> MSDNRRRRREEDDSDSENELPPSSPQQHFRGGMNPVSSPIGSPDMINPEGDDNEVDDVPDIDEVEEQMNEVDLMDDNMYEDYAADHNRDRYDPDQVDDREQQELSLSERRRIDAQLNERDRLLRNVAYIDDEDEEQEGAAQLDEMGLPVQRRRRRRQYEDLENSDDDLLSDMDIDPLREELTLESLSNVKANSYSEWITQPNVSRTIARELKSFLLEYTDETGRSVYGARIRTLGEMNSESLEVNYRHLAESKAILALFLAKCPEEMLKIFDLVAMEATELHYPDYARIHSEIHVRISDFPTIYSLRELRESNLSSLVRVTGVVTRRTGVFPQLKYVKFNCLKCGSILGPFFQDSNEEIRISFCTNCKSKGPFRVNGEKTVYRNYQRVTLQEAPGTVPPGRLPRHREVILLADLVDVSKPGEEVEVTGIYKNNYDGNLNAKNGFPVFATIIEANSIKRREGNTANEGEEGLDVFSWTEEEEREFRKISRDRGIIDKIISSMAPSIYGHRDIKTAVACSLFGGVPKNVNGKHSIRGDINVLLLGDPGTAKSQILKYVEKTAHRAVFATGQGASAVGLTASVRKDPITKEWTLEGGALVLADKGVCLIDEFDKMNDQDRTSIHEAMEQQSISISKAGIVTTLQARCSIIAAANPNGGRYNSTLPLAQNVSLTEPILSRFDILCVVRDLVDEEADERLATFVVDSHVRSHPENDEDREGEELKNNGESAIEQGEDEINEQLNARQRRLQRQRKKEEEISPIPQELLMKYIHYARTKIYPKLHQMDMDKVSRVYADLRRESISTGSFPITVRHLESILRIAESFAKMRLSEFVSSYDLDRAIKVVVDSFVDAQKVSVRRQLRRSFAIYTLGH;> MKRRWKKNFIAVSAANRFKKISSSGALENLYFQGEA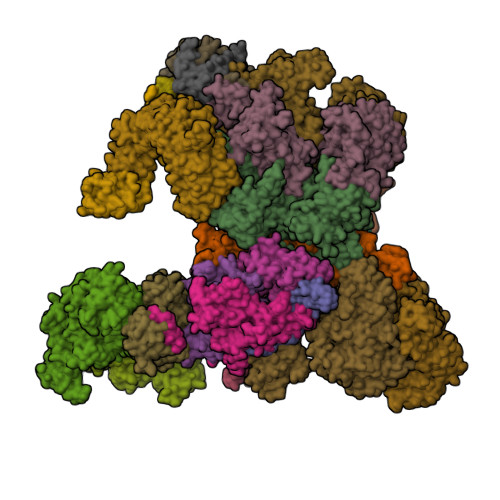PVMEGSTGFDGDATTFFAPDAVFGDRVRRFQEFLDTFTSYRDSVRSIQVYNSNNAANYNDDQDDADERDLLGDDDGDDLEKEKKAASSTSLNILPHRIIISLDDLREFDRSFWSGILVEPAYFIPPAEKALTDLADSMDDVPHPNASAVSSRHPWKLSFKGSFGAHALSPRTLTAQHLNKLVSVEGIVTKTSLVRPKLIRSVHYAAKTGRFHYRDYTDATTTLTTRIPTPAIYPTEDTEGNKLTTEYGYSTFIDHQRITVQEMPEMAPAGQLPRSIDVILDDDLVDKTKPGDRVNVVGVFKSLGAGGMNQSNSNTLIGFKTLILGNTVYPLHARSTGVAARQMLTDFDIRNINKLSKKKDIFDILSQSLAPSIYGHDHIKKAILLMLMGGVEKNLENGSHLRGDINILMVGDPSTAKSQLLRFVLNTASLAIATTGRGSSGVGLTAAVTTDRETGERRLEAGAMVLADRGVVCIDEFDKMTDVDRVAIHEVMEQQTVTIAKAGIHTTLNARCSVIAAANPVFGQYDVNRDPHQNIALPDSLLSRFDLLFVVTDDINEIRDRSISEHVLRTHRYLPPGYLEGEPVRERLNLSLAVGEDADINPEEHSNSGAGVENEGEDDEDHVFEKFNPLLQAGAKLAKNKGNYNGTEIPKLVTIPFLRKYVQYAKERVIPQLTQEAINVIVKNYTDLRNDDNTKKSPITARTLETLIRLATAHAKVRLSKTVNKVDAKVAANLLRFALLGEDIGNDIDEEESEYEEALSKRSPQKSPKKRQRVRQPASNSGSPIKSTPRRSTASSVNATPSSARRILRFQDDEQNAGEDDNDIMSPLPADEEAELQRRLQLGLRVSPRRREHLHAPEEGSSGPLTEVGTPRLPNVSSAGQDDEQQQSVISFDNVEPGTISTGRLSLISGIIARLMQTEIFEEESYPVASLFERINEELPEEEKFSAQEYLAGLKIMSDRNNLMVADDKVWRV;> MSQQSSSPTKEDNNSSSPVVPNPDSVPPQLSSPALFYSSSSSQGDIYGRNNSQNLSQGEGNIRAAIGSSPLNFPSSSQRQNSDVFQSQGRQGRIRSSASASGRSRYHSDLRSDRALPTSSSSLGRNGQNRVHMRRNDIHTSDLSSPRRIVDFDTRSGVNTLDTSSSSAPPSEASEPLRIIWGTNVSIQECTTNFRNFLMSFKYKFRKILDEREEFINNTTDEELYYIKQLNEMRELGTSNLNLDARNLLAYKQTEDLYHQLLNYPQEVISIMDQTIKDCMVSLIVDNNLDYDLDEIETKFYKVRPYNVGSCKGMRELNPNDIDKLINLKGLVLRSTPVIPDMKVAFFKCNVCDHTMAVEIDRGVIQEPARCERIDCNEPNSMSLIHNRCSFADKQVIKLQETPDFVPDGQTPHSISLCVYDELVDSCRAGDRIEVTGTFRSIPIRANSRQRVLKSLYKTYVDVVHVKKVSDKRLDVDTSTIEQELMQNKVDHNEVEEVRQITDQDLAKIREVAAREDLYSLLARSIAPSIYELEDVKKGILLQLFGGTNKTFTKGGRYRGDINILLCGDPSTSKSQILQYVHKITPRGVYTSGKGSSAVGLTAYITRDVDTKQLVLESGALVLSDGGVCCIDEFDKMSDSTRSVLHEVMEQQTISIAKAGIITTLNARSSILASANPIGSRYNPNLPVTENIDLPPPLLSRFDLVYLVLDKVDEKNDRELAKHLTNLYLEDKPEHISQDDVLPVEFLTMYISYAKEHIHPIITEAAKTELVRAYVGMRKMGDDSRSDEKRITATTRQLESMIRLAEAHAKMKLKNVVELEDVQEAVRLIRSAIKDYATDPKTGKIDMNLVQTGKSVIQRKLQEDLSREIMNVLKDQASDSMSFNELIKQINEHSQDRVESSDIQEALSRLQQEDKVIVLGEGVRRSVRLNNRV;> MSFDRPEIYSAPVLQGESPNDDDNTEIIKSFKNFILEFRLDSQFIYRDQLRNNILVKNYSLTVNMEHLIGYNEDIYKKLSDEPSDIIPLFETAITQVAKRISILSRAQSANNNDKDPENTSMDTDSLLLNSLPTFQLILNSNANQIPLRDLDSEHVSKIVRLSGIIISTSVLSSRATYLSIMCRNCRHTTSITINNFNSITGNTVSLPRSCLSTIESESSMANESNIGDESTKKNCGPDPYIIIHESSKFIDQQFLKLQEIPELVPVGEMPRNLTMTCDRYLTNKVIPGTRVTIVGIYSIYNSKNGAGSGRSGGGNGGSGVAIRTPYIKILGIQSDVETSSIWNSVTMFTEEEEEEFLQLSRNPKLYEILTNSIAPSIFGNEDIKKAIVCLLMGGSKKILPDGMRLRGDINVLLLGDPGTAKSQLLKFVEKVSPIAVYTSGKGSSAAGLTASVQRDPMTREFYLEGGAMVLADGGVVCIDEFDKMRDEDRVAIHEAMEQQTISIAKAGITTVLNSRTSVLAAANPIYGRYDDLKSPGDNIDFQTTILSRFDMIFIVKDDHNEERDISIANHVINIHTGNANAMQNQQEENGSEISIEKMKRYITYCRLKCAPRLSPQAAEKLSSNFVTIRKQLLINELESTERSSIPITIRQLEAIIRITESLAKLELSPIAQERHVDEAIRLFQASTMDAASQDPIGGLNQASGTSLSEIRRFEQELKRRLPIGWSTSYQTLRREFVDTHRFSQLALDKALYALEKHETIQLRHQGQNIYRSGV;> MSSPFPADTPSSNRPSNSSPPPSSIGAGFGSSSGLDSQIGSRLHFPSSSQPHVSNSQTGPFVNDSTQFSSQRLQTDGSATNDMEGNEPARSFKSRALNHVKKVDDVTGEKVREAFEQFLEDFSVQSTDTGEVEKVYRAQIEFMKIYDLNTIYIDYQHLSMRENGALAMAISEQYYRFLPFLQKGLRRVVRKYAPELLNTSDSLKRSEGDEGQADEDEQQDDDMNGSSLPRDSGSSAAPGNGTSAMATRSITTSTSPEQTERVFQISFFNLPTVHRIRDIRSEKIGSLLSISGTVTRTSEVRPELYKASFTCDMCRAIVDNVEQSFKYTEPTFCPNPSCENRAFWTLNVTRSRFLDWQKVRIQENANEIPTGSMPRTLDVILRGDSVERAKPGDRCKFTGVEIVVPDVTQLGLPGVKPSSTLDTRGISKTTEGLNSGVTGLRSLGVRDLTYKISFLACHVISIGSNIGASSPDANSNNRETELQMAANLQANNVYQDNERDQEVFLNSLSSDEINELKEMVKDEHIYDKLVRSIAPAVFGHEAVKKGILLQMLGGVHKSTVEGIKLRGDINICVVGDPSTSKSQFLKYVVGFAPRSVYTSGKASSAAGLTAAVVRDEEGGDYTIEAGALMLADNGICCIDEFDKMDISDQVAIHEAMEQQTISIAKAGIHATLNARTSILAAANPVGGRYNRKLSLRGNLNMTAPIMSRFDLFFVILDDCNEKIDTELASHIVDLHMKRDEAIEPPFSAEQLRRYIKYARTFKPILTKEARSYLVEKYKELRKDDAQGFSRSSYRITVRQLESMIRLSEAIARANCVDEITPSFIAEAYDLLRQSIIRVDVDDVEMDEEFDNIESQSHAASGNNDDNDDGTGSGVITSEPPADIEEGQSEATARPGTSEKKKTTVTYDKYVSMMNMIVRKIAEVDREGAEELTAVDIVDWYLLQKENDLGSLAEYWEERRLAFKVIKRLVKDRILMEIHGTRHNLRDLENEENENNKTVYVIHPNCEVLDQLEPQDSS;> MSAALPSIQLPVDYNNLFNEITDFLVTFKQDTLSSDATRNENEDENLDAENIEQHLLEKGPKYMAMLQKVANRELNSVIIDLDDILQYQNEKFLQGTQADDLVSAIQQNANHFTELFCRAIDNNMPLPTKEIDYKDDVLDVILNQRRLRNERMLSDRTNEIRSENLMDTTMDPPSSMNDALREVVEDETELFPPNLTRRYFLYFKPLSQNCARRYRKKAISSKPLSVRQIKGDFLGQLITVRGIITRVSDVKPAVEVIAYTCDQCGYEVFQEVNSRTFTPLSECTSEECSQNQTKGQLFMSTRASKFSAFQECKIQELSQQVPVGHIPRSLNIHVNGTLVRSLSPGDIVDVTGIFLPAPYTGFKALKAGLLTETYLEAQFVRQHKKKFASFSLTSDVEERVMELITSGDVYNRLAKSIAPEIYGNLDVKKALLLLLVGGVDKRVGDGMKIRGDINVCLMGDPGVAKSQLLKAICKISPRGVYTTGKGSSGVGLTAAVMKDPVTDEMILEGGALVLADNGICCIDEFDKMDESDRTAIHEVMEQQTISISKAGINTTLNARTSILAAANPLYGRYNPRLSPLDNINLPAALLSRFDILFLMLDIPSRDDDEKLAEHVTYVHMHNKQPDLDFTPVEPSKMREYIAYAKTKRPVMSEAVNDYVVQAYIRLRQDSKREMDSKFSFGQATPRTLLGIIRLSQALAKLRLADMVDIDDVEEALRLVRVSKESLYQETNKSKEDESPTTKIFTIIKKMLQETGKNTLSYENIVKTVRLRGFTMLQLSNCIQEYSYLNVWHLINEGNTLKFVDDGTMDTDQEDSLVSTPKLAPQTTASANVSAQDSDIDLQDA;> MYGDLGNKLVLEAKRTKQLYARSNQDVNLPMYHEDIIRNILKEVSNLRKNTEYLKEQQQLGMLDDKVAKCQYFVTLLCMERNKRCLLAYQRLRTDILDSMAWNNNGLDLMSSITFSQQDTNNLSHQEQEYLKEYCDLITDLKSGDLVDIDLSGSLVPPSDVFIDVRVLKDAGEIQTEYGVFNLIKDSQFFVRQSDVERLIQQGYLQKI;> MSLPAHLQQTFSPEEIQFIVENEPIKIFPRITTRQKIRGDDRGTGNHTRWQLITTDDKALNNMVAMRSTEVVLWIALLLKQQSKCSIVAPQWLTTKELDRKIQYEKTHPDRFSELPWNWLVLARILFNKAKDDFHDPIHELRGKIQDLREIRQIKVLKGLKYLNESHLQLDNLSLLEINELRPFITEIMDKLREIHTASLTAGTENDEEEFNI;> MGYYDIDDVLADGTEFPCKFQYDIPGLGYLENNPGRPITKNTKLNLPLWLARILAIVGGDEALVDEEPVPFVELLPPDMFSTKVMNAIKTDPVALDLHSINSHFFSLAIKWIMLFSEKELANVVSELLLQRAQELNHHASSLSIDLNADSTGKNSANTNIATSTFLLKLEEMEKEIYKKSHESYKDTKRWMFKK;> MDINIDDILAELDKETTAVDSTKITQGSSSTTHRDANTIVGSSLDLNDKTQIYVSPQQDFSDLMKSWKNERCSPELLPYPHQLMKRLLNRISMQSQLIENISMGFLDMQNASNANPPMPNESKLPLLCMETELERLKFVIRSYIRCRLSKIDKFSLYLRQLNEDENSLISLTDLLSKDEIKYHDTHSLIWLKLVNDSILKYMPEELQAINDTEGSVNMIDEPDWNKFVFIHVNGPPDGKWNEDPLLQENEFGKPCYTVTIPDLKEEVELTIGSIYVMRYEVIRDLLRDDKVALI;> MYYGISQFSEAYNKILRNSSSHSSCQLVIFVSCLNIDALCATKMLSLLFKKQLVQSQIVPIFGYSELRRHYSQLDDNINSLLLVGFGGVIDLEAFLEIDPQEYVIDTDEKSGEQSFRRDIYVLDAHRPWNLDNIFGSQIIQCFDDGTVDDTLGEQKEAYYKLLELDEESGDDELSGDENDNNGGDDEATDADEVTDEDYKDDDGDYKDDDETISNKRGNSSIGPNDLSKRKQRKKQIHEYEGVLEEYYSQGTTVVNSISAQIYSLLSAIGETNLSNLWLNILGTTSLDIAYAQVYNRLYPLLQDEVKRLTPSSRNSVKTPDTLTLNIQPDYYLFLLRHSSLYDSFYYSNYVNAKLSLWNENGKKRLHKMFARMGIPLSTAQETWLYMDHSIKRELGIIFDKNLDRYGLQDIIRDGFVRTLGYRGSISASEFVEALTALLEVGNSTDKDSVKINNDNNDDTDGEEEEDNSAQKLTNLRKRWVSNFWLSWDALDDRKVELLNRGIQLAQDLQRAIFNTGVAILEKKLIKHLRIYRLCVLQDGPDLDLYRNPLTLLRLGNWLIECCAESEDKQLLPMVLASIDENTDTYLVAGLTPRYPRGLDTIHTKKPILNNFSMAFQQITAETDAKVRIDNFESSIIEIRREDLSPFLEKLTLSGLL;>[3x]MKRRWKKNFIAVSAANRFKKISSSGALENLYFQGEMVSVIDKLVFDFGGKTLVSLAPDNNTLCVANKNGLTKILKTNNPEEEPETLDSSKLVSSIKCYSNSHFLMTTMQGDALRYNIDSSQEELLARFALPLRDCCVIHSGKMAVFGGDDLELILLELDDETHKKHAIKIDEQVSQISYNSQMNILAVSMINGKVQIFSLTSTIPNKVHELNDYIVANSYDDTHRDKILSNMMDDIDKDNDNDLSETADPDENNVADPEFCAANRICTRVAWHPKGLHFALPCADDTVKIFSIKGYSLQKTLSTNLSSTKAHFIDLQFDPLRGTYIAAVDLNNKLTVWNWETSEIHYTREFKRKITNIAWKIQADSKTLDLVLGTWSGSIAIVQNLAESVVSNIPDQSVAESSTKHGLFVDSESDLENLEGNDDINKSDKLFSDITQEANAEDVFTQTHDGPSGLSEKRKYNFEDEEDFIDDDDGAGYISGKKPHNEHSYSRVHKTHSFPISLANTGKFRYMPFSPAGTPFGFTDRRYLTMNEVGYVSTVKNSEQYSITVSFFDVGRFREYHFEDLFGYDLCFLNEKGTLFGQSKTGQIQYRPHDSIHSNWTKIIPLQAGERITSVAATPVRVIVGTSLGYFRSFNQFGVPFAVEKTSPIVALTAQNYRVFSVHYSQFHGLSYSLSELGTSSKRYYKRECPLPMSLPNINSDMKKDANLDYYNFNPMGIKSLFFSSYGDPCIFGSDNTLLLLSKWRSPEESKWLPILDSNMEIWKMSGGKETTDIHVWPLALAYDTLNCILVKGKHIWPEFPLPLPSEMEIRMPVFVKSKLLEENKAILNKKNEIGADTEAEEGEEDKEIQIPVSMAAEEEYLRSKVLSELLTDTLENDGEMYGNENEVLAALNGAYDKALLRLFASACSDQNVEKALSLAHELKQDRALTAAVKISERAELPSLVKKINNIREARYEQQLK;> MVTSNVVLVSGEGERFTVDKKIAERSLLLKNYLNDMHDSNLQNNSDSESDSDSETNHKSKDNNNGDDDDEDDDEIVMPVPNVRSSVLQKVIEWAEHHRDSNFPDEDDDDSRKSAPVDSWDREFLKVDQEMLYEIILAANYLNIKPLLDAGCKVVAEMIRGRSPEEIRRTFNIVNDFTPEEEAAIRRENEWAEDR;> GAGMSSPGNSGVAIDSTVLKAIELGTRLFKSGEYLQAKRIFTNALRVCDSYSQEQIMRIRNAYQLDTARPDNKRLYHPRYIKILDNICACYEKLNDLKSCLDVSQRLLKLEPGNIKCYIRCTRTLIKLKDWKRAYKTCSRGLQLCNNDSNHLRQQKQFIKNNMVQKQDGKRSYIDPLEETKIAKKKKNNNVLESLPKKKIKGSTKKTDLVGNLPIEILPIIFQRFTTKELVTLSLVCNKWRDKILYHLDCFQEFNLAPINFKNFVKFMDFLQQNFTRTYRKYILSQVKVSSRITSEELRITQLLFSKMPKCINIERLILSMPTLTTTQIFKLMVRGGTDFFTRLLELSLMITYRPDKQHELEILQTCPLLKKIELIFVNSLVPIFDGNNSVGRDGSFNVMARHTNMQISTADNDEQGIVEEKVIYSELEKITLICDKKKIKNFPLCRALLRGQFPLLQKLTITGVTFPMNNQDIMNFQWLLNFPDLKELWIEDNDNCELSKFLQLLKFSNVWKNLEKLTFRENKLYPIVNLDEDQPVTNDDEVPSMLFYKENLQNLEKLDLMGTSISGSALTRLCEQEYLDGRKLRSLNIGNCPNIQFPNNHAHTARMILDVNAVLKRLSKLEEINLSHLSSLNDSTMKSFIINVPFLENLKRLDISHNFEITGISIYEFLKKFQMDHDNEAGGQPLAYLNIDGCSQVSHITVNMIRAQNLVTQVDCVYERDVWRKFGINSYSYS;> MMFGKKKNNGGSSTARYSAGNKYNTLSNNYALSAQQLLNASKIDDIDSMMGFERYVPPQYNGRFDAKDIDQIPGRVGWLTNMHATLVSQETLSSGSNGGGNSNDGERVTTNQGISGVDFYFLDEEGGSFKSTVVYDPYFFIACNDESRVNDVEELVKKYLESCLKSLQIIRKEDLTMDNHLLGLQKTLIKLSFVNSNQLFEARKLLRPILQDNANNNVQRNIYNVAANGSEKVDAKHLIEDIREYDVPYHVRVSIDKDIRVGKWYKVTQQGFIEDTRKIAFADPVVMAFAIATTKPPLKFPDSAVDQIMMISYMIDGEGFLITNREIISEDIEDFEYTPKPEYPGFFTIFNENDEVALLQRFFEHIRDVRPTVISTFNGDFFDWPFIHNRSKIHGLDMFDEIGFAPDAEGEYKSSYCSHMDCFRWVKRDSYLPQGSQGLKAVTQSKLGYNPIELDPELMTPYAFEKPQHLSEYSVSDAVATYYLYMKYVHPFIFSLCTIIPLNPDETLRKGTGTLCEMLLMVQAYQHNILLPNKHTDPIERFYDGHLLESETYVGGHVESLEAGVFRSDLKNEFKIDPSAIDELLQELPEALKFSVEVENKSSVDKVTNFEEIKNQITQKLLELKENNIRNELPLIYHVDVASMYPNIMTTNRLQPDSIKAERDCASCDFNRPGKTCARKLKWAWRGEFFPSKMDEYNMIKRALQNETFPNKNKFSKKKVLTFDELSYADQVIHIKKRLTEYSRKVYHRVKVSEIVEREAIVCQRENPFYVDTVKSFRDRRYEFKGLAKTWKGNLSKIDPSDKHARDEAKKMIVLYDSLQLAHKVILNSFYGYVMRKGSRWYSMEMAGITCLTGATIIQMARALVERVGRPLELDTDGIWCILPKSFPETYFFTLENGKKLYLSYPCSMLNYRVHQKFTNHQYQELKDPLNYIYETHSENTIFFEVDGPYKAMILPSSKEEGKGIKKRYAVFNEDGSLAELKGFELKRRGELQLIKNFQSDIFKVFLEGDTLEGCYSAVASVCNRWLDVLDSHGLMLEDEDLVSLICENRSMSKTLKEYEGQKSTSITTARRLGDFLGEDMVKDKGLQCKYIISSKPFNAPVTERAIPVAIFSADIPIKRSFLRRWTLDPSLEDLDIRTIIDWGYYRERLGSAIQKIITIPAALQGVSNPVPRVEHPDWLKRKIATKEDKFKQTSLTKFFSKTKNVPTMGKIKDIEDLFEPTVEEDNAKIKIARTTKKKAVSKRKRNQLTNEEDPLVLPSEIPSMDEDYVGWLNYQKIKWKIQARDRKRRDQLFGNTNSSRERSALGSMIRKQAESYANSTWEVLQYKDSGEPGVLEVFVTINGKVQNITFHIPKTIYMKFKSQTMPLQKIKNCLIEKSSASLPNNPKTSNPAGGQLFKITLPESVFLEEKENCTSIFNDENVLGVFEGTITPHQRAIMDLGASVTFRSKAMGALGKGIQQGFEMKDLSMAENERYLSGFSMDIGYLLHFPTSIGYEFFSLFKSWGDTITILVLKPSNQAQEINASSLGQIYKQMFEKKKGKIETYSYLVDIKEDINFEFVYFTDISKLYRRLSQETTKLKEERGLQFLLLLQSPFITKLLGTIRLLNQMPIVKLSLNEVLLPQLNWQPTLLKKLVNHVLSSGSWISHLIKLSQYSNIPICNLRLDSMDYIIDVLYARKLKKENIVLWWNEKAPLPDHGGIQNDFDLNTSWIMNDSEFPKINNSGVYDNVVLDVGVDNLTVNTILTSALINDAEGSDLVNNNMGIDDKDAVINSPSEFVHDAFSNDALNVLRGMLKEWWDEALKENSTADLLVNSLASWVQNPNAKLFDGLLRYHVHNLTKKALLQLVNEFSALGSTIVYADRNQILIKTNKYSPENCYAYSQYMMKAVRTNPMFSYLDLNIKRYWDLLIWMDKFNFSGLACIEIEEKENQDYTAVSQWQLKKFLSPIYQPEFEDWMMIILDSMLKTKQSYLKLNSGTQRPTQIVNVKKQDKEDSVENSLNGFSHLFSKPLMKRVKKLFKNQQEFILDPQYEADYVIPVLPGSHLNVKNPLLELVKSLCHVMLLSKSTILEIRTLRKELLKIFELREFAKVAEFKDPSLSLVVPDFLCEYCFFISDIDFCKAAPESIFSCVRCHKAFNQVLLQEHLIQKLRSDIESYLIQDLRCSRCHKVKRDYMSAHCPCAGAWEGTLPRESIVQKLNVFKQVAKYYGFDILLSCIADLTI;> MFGSGNVLPVKIQPPLLRPLAYRVLSRKYGLSIKSDGLSALAEFVGTNIGANWRQGPATIKFLEQFAAVWKQQERGLFIDQSGVKEVIQEMKEREKVEWSHEHPIQHEENILGRTDDDENNSDDEMPIAADSSLQNVSLSSPMRQPTERDEYKQPFKPESSKALDWRDYFKVINASQQQRFSYNPHKMQFIFVPNKKQNGLGGIAGFLPDIEDKVQMFLTRYYLTNDRVMRNENFQNSDMFNPLSSMVSLQNELSNTNRQQQSSSMSITPIKNLLGRDAQNFLLLGLLNKNFKGNWSLEDPSGSVEIDISQTIPTQGHYYVPGCMVLVEGIYYSVGNKFHVTSMTLPPGERREITLETIGNLDLLGIHGISNNNFIARLDKDLKIRLHLLEKELTDHKFVILGANLFLDDLKIMTALSKILQKLNDDPPTLLIWQGSFTSVPVFASMSSRNISSSTQFKNNFDALATLLSRFDNLTENTTMIFIPGPNDLWGSMVSLGASGTLPQDPIPSAFTKKINKVCKNVVWSSNPTRIAYLSQEIVIFRDDLSGRFKRHRLEFPFNESEDVYTENDNMMSKDTDIVPIDELVKEPDQLPQKVQETRKLVKTILDQGHLSPFLDSLRPISWDLDHTLTLCPIPSTMVLCDTTSAQFDLTYNGCKVINPGSFIHNRRARYMEYVPSSKKTIQEEIYI;> MSADLQQGTTNAADFSLTVLRARIALLATAIGGPDYTSQIDPPPYKLGDDCLACLKDLKRWFKLVDDQQKRWDVAMAVAEYRILTDDLLPILIDWENKCSLAAKLAKNNPDHEEFRNKAYYDKIALNCLQLLVLMTWPLIVTEQSSSNQITLYGELKKHQLVYKKTILSMESGKVLRAAIRLALDVIKIDRLSRTPRDNMVLKLVLNFFRNVIAIEPGEFTINTKKSMPKKGITSIDTLPPNVSMDDISLNTVISSFHKNKVFGFLLTLTSSLSKEFDQDFINIPLLEIMFYFTKDVNQELLFPRQFETGTHSKVVNKNESSSANNIVTSAGFELSKLLQKEHQMRKNVIKHTSARHSRFGGLLSIQTPDKTRLTVSGSQALVDEKIALQKLDDSKKWNKRIIKKHQSVAAEGLPNSLLNSQTGKAIFFTESNGKHFKEFINNFIDSGFNILLHSVTNYFTTEQDRMVTLEQVEYLLFFAWFVKYQLLRSKIDNSADIKQVSEALKEVTFILVSSLLRSAYDLKNWTVTHAGMIAFNELLNLVSRTKAAQEEDSTDIEFIVSRLFSDERIQLLSNLPKIGSKYSLQFMKSCIELTHSVLKVLEQYSDDKTLVIEGKSRRQKKFNISEGDITKLIEEENVDRDEALDILTSSLRSIEVNFQKVQANYMTEPVIETYINFLERFRELEDDSIKKVFSFFHRVFVQAKEQALLFRFDLIILLREMLSPDGLDRMSRSRKYVSQFSDYFLARLKKRLKKSPAWFVGLLFPPLHNSEVGFYQRYGEYNVLNNESMYAAPASQFKPIPDEEALPPSILLDMKYGVLVSTLLDDGKTELLDQLLKHITHTLDIFKSWLTVNVNAGKETVNPPNEYFTLTGVLNNDPIFKDKDYRALLLLIGYSIPRKINEPCFLPGTVEVSDLTVSCELVKKYLSTPFETPNGLPSSSYLLRVRSEKDSFSHNEQDGWEGDDDYDYNDPYIVPDDQILSKSDAAYFKDLDNNASDKLKGTKFSKGIARSKKKDKRKRRKGEAKTNLPMFGDQDDERPQTVRERHGVFSKEFISDSEDDEDLMNPIFFENETYMRWLLDKNNGQLTEDRYIQFAKFAAERMNNGGVVTGDYTSLFGGSIPSIESIRATESSSFAPDKSLISLASHVASEMSIFDVNNNNNNQLSDDDVNSESRNSLGSSQPSNSQNMFQSEVYSRKESTKRSLEASAADESDEDEEAIRLFGKKSRVVLSQGDSDD;> GEMDQDFDSLLLGFNDSDSVQKDPTVPNGLDGSVVDPTIADPTAITARKRRPQVKLTAEKLLSDKGLPYVLKNAHKRIRISSKKNSYDNLSNIIQFYQLWAHELFPKAKFKDFMKICQTVGKTDPVLREYRVSLFRDEMGMSFDVGTRETGQDLERQSPMVEEHVTSAEERPIVADSFAQDKRNVNNVDYDNDEDDDIYHLSYRNRRGRVLDERGNNETVLNNVVPPKEDLDALLKTFRVQGPVGLEENEKKLLLGWLDAHRKMEKGSMTEEDVQLIQSLEEWEMNDIEGQHTHYDLLPGGDEFGVDQDELDAMKEMGF> AAGSHMAAEYKFPDPIPEFAEAETEKFRDHMLNKLSKRDLFEDSV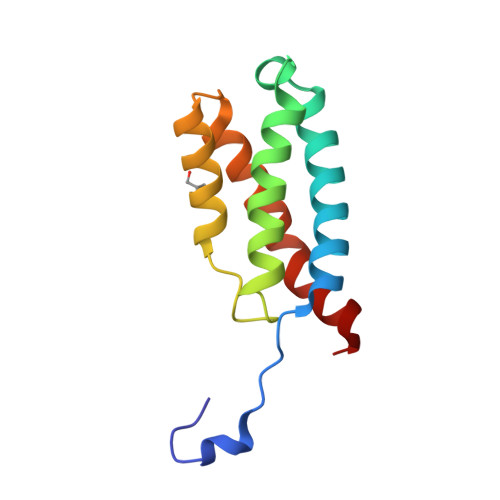DEIVGVCTEIFETFLRSEYGGPGTLLVIPFIDMADTLNERELPGGPQAARAAIKWAQDHVDKDWKEWTGT>MSMNRQEISDLCVKSLEGRMVGTEAQNIENGNAFYRYFFTNFPDLRVYFKGAEKYTADDVKKSERFDKQGQRILLACHLLANVYTNEEVFKGYVRETINRHRIYKMDPALWMAFFTVFTGY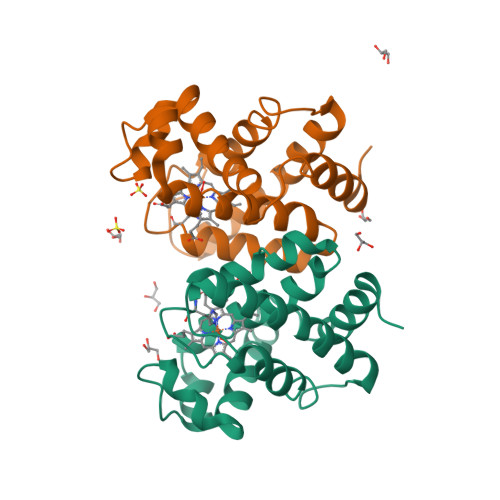LESVGSLNDQQKAAWMALGKEFNAESQTHLKNSNLPHV[2x]>[2x]HHHHHHSSGLVPRGSHMQSMRFMILALLVQFLPAWAINDPAKSAAPYHDEFPLFRSANMASPDKLSTGIGFHSFRIPAVVRTTTGRILAFAEGRRHTNQDFGDINLVYKRTKTTANNGASPSDWEPLREVVGSGAGTWGNPTPVVDDDNTIYLFLSWNGATYSQNGKDVLPDGTVTKKIDSTWEGRRH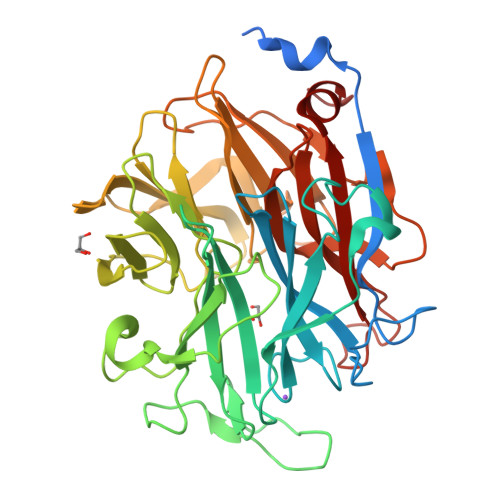LYLTESRDDGNTWSKPVDLTKELTPDGWAWDAVGPGNGIRLTTGELVIPAMGRNIIGRGAPGNRTWSVQRLSGAGAEGTIVQTPDGKLYRNDRPSQKGYRMVARGTLEGFGAFAPDAGLPDPACQGSVLRYNSDAPARTIFLNSASGTSRRAMRVRISYDADAKKFNYGRKLEDAKVSGAGHEGGHSSMTKTGDYKIGALVESDFFNDGTGKNSYRAIIWRRFNLSWILNGPNN[azanyl(thiophen-3-yl)methylidene]azanium | C5 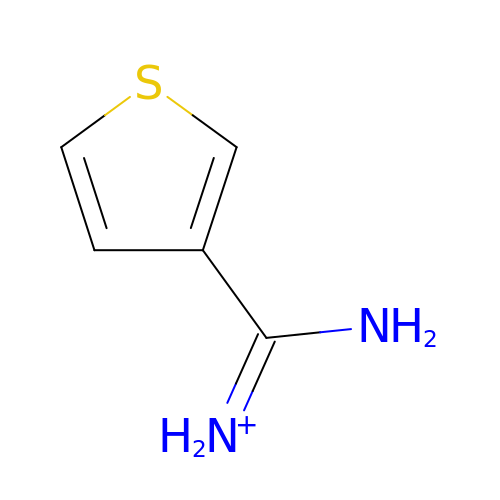H7 N2 S | JKCKRNYECSTMLV-UHFFFAOYSA-O> NAMYTITDIAPTDAEFIALIAALDAWQETLYPAESNHLLDLS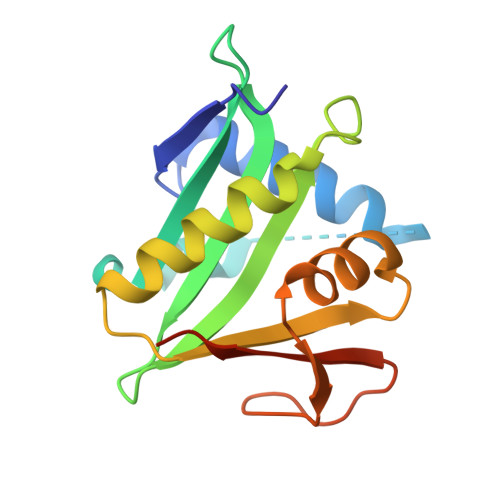QLPPQTVIALAIRSPQGEAVGCGAIVLSEEGFGEMKRVYIDPQHRGQQLGEKLLAALEAKARQRDCHTLRLETGIHQHAAIALYTRNGYQTRCAFAPYQPDPLSVFMEKPLFADLRSAAL>GAMEGFKANLSLLRRPGEKTYTQRCRLFVGNLPADITEDEFKRLFAKYGEPGEVFINKGKGFGFIKLESRALAEIAKAELDDTPMRGRQLRVRFATHAAALSVRNLSPYVSNELLEEAFSQFGPIERAVVIVDDRGRSTGKGI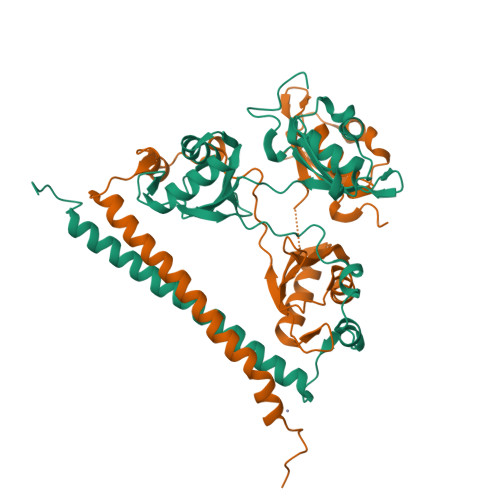VEFASKPAARKAFERCSEGVFLLTTTPRPVIVEPLEQLDDEDGLPEKLAQKNPMYQKERETPPRFAQHGTFEYEYSQRWKSLDEMEKQQREQVEKNMKDAKDKLESEMEDAYHEHQANLL[2x]[[(2R,3S,4R,5R)-5-(6-aminopurin-9-yl)-4-oxidanyl-3-phosphonooxy-oxolan-2-yl]methoxy-oxidanyl-phosphoryl] 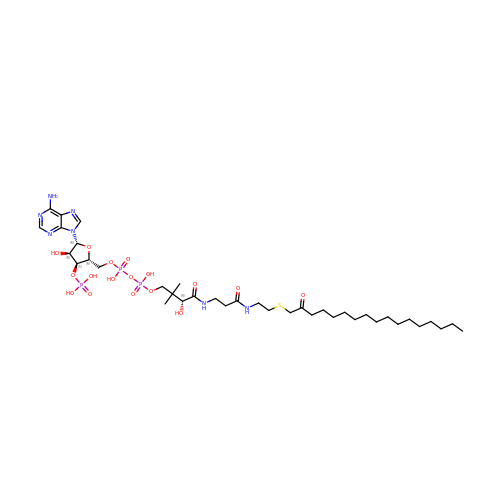[(3R)-2,2-dimethyl-3-oxidanyl-4-oxidanylidene-4-[[3-oxidanylidene-3-[2-(2-oxidanylideneheptadecylsulfanyl)ethylamino]propyl]amino]butyl] hydrogen phosphate | C38 H68 N7 O17 P3 S | SBIFJLISRCXPBF-QYIYCXJMSA-N> MLKQVEIFTDGSCLGNPGPGGYGAILRYRGREKTFSAGYTRTTNNRMELMAAIVALEALKEHCEVILSTDSQYVRQGITQWIHNWKK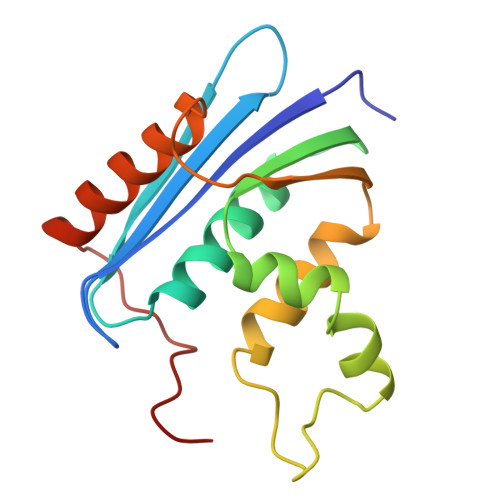RGWKTADKKPVKNVDLWQRLDAALGQHQIKWEWVKGHAGHPENERCNELARAAAMNPTLEDTGYQVEV>MQKPVCLVVAMTPKRGIGINNGLPWPHLTTDFKHFSRVTKTTPEEASRFNAVVMGRKTWESMPRKFRPLVDRLNIVVSSSLKEEDIAAEKPQAEGQQRVRVCASLPAALSLLEEEYKDSVDQIFVVGGAGLYEAALSLGVASHLYITRVAREFPCDVFFPAFPGDDILSNKSTAAEKDNEATYRPIFISKTFSDNGVPYDFV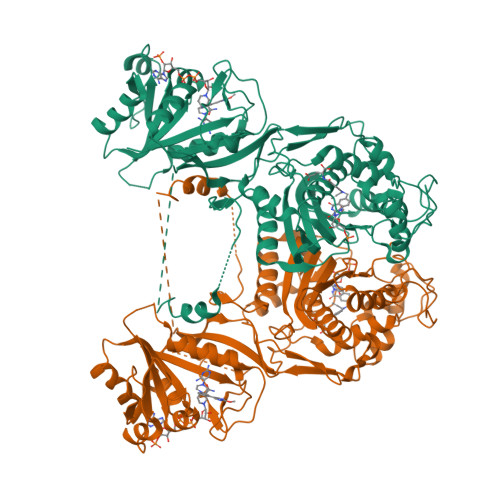VLEKRRKTDDAATAEPSNAMSSLTSTRETTPVHGLQAPSSAAAIAPVLAWMDEEDRKKREQKELIRAVPHVHFRGHEEFQYLDLIADIINNGRTMDDRTGVGVISKFGCTMRYSLDQAFPLLTTKRVFWKGVLEELLWFIRGDTNANHLSEKGVKIWDKNVTREFLDSRNLPHREVGDIGPGYGFQWRHFGAAYKDMHTDYTGQGVDQLKNVIQMLRTNPTDRRMLMTAWNPAALDEMALPPCHLLCQFYVNDQKELSCIMYQRSCDVGLGVPFNIASYSLLTLMVAHVCNLKPKEFIHFMGNTHVYTNHVEALKEQLRREPRPFPIVNILNKERIKEIDDFTAEDFEVVGYVPHGRIQMEMAV[2x]>SNAALSQSGPDGLASITLPLPISAERGFAPALALHYSSGGGNGPFGVGWSCATMSIARRTSHGVPQYNDSDEFLGPDGEVLVQTLSTGDAPNPVTCFAYGDVSFPQSYTVTRYQ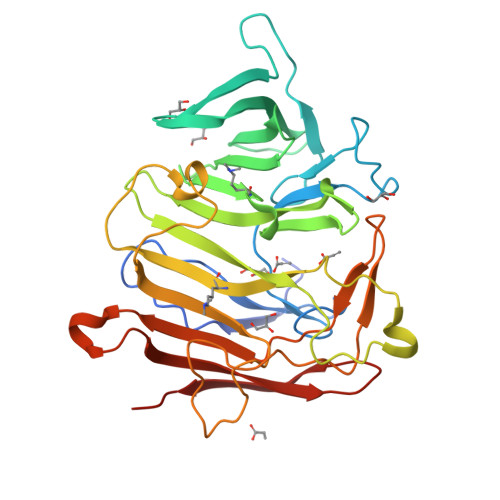PRTESSFYRLEYWVGNSNGDDFWLLHDSNGILHLLGKTAAARLSDPQAASHTAQWLVEESVTPAGEHIYYSYLAENGDNVDLNGNEAGRDRSAMRYLSKVQYGNATPAADLYLWTSATPAVQWLFTLVFDYGERGVDPQVPPAFTAQNSWLARQDPFSLYNYGFEIRLHRLCRQVLMFHHFPDELGEADTLVSRLLLEYDENPILTQLCAARTLAYEGD[2x]4-(7-azanyl-5,5-dimethyl-3-methylimino-benzo[b][1]benzosilin-10-yl)-N-[2-[2-(6-chloranylhexoxy)ethoxy]ethyl]-3-methyl-benzamide 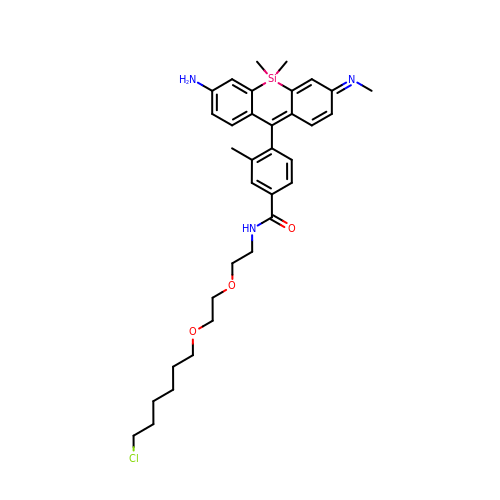| C34 H44 Cl N3 O3 Si | JCDPTWLYDNGHLA-NXEFEZKASA-N> MSRGRKNNDIPLSFYNPITLEQGSKFWNLCP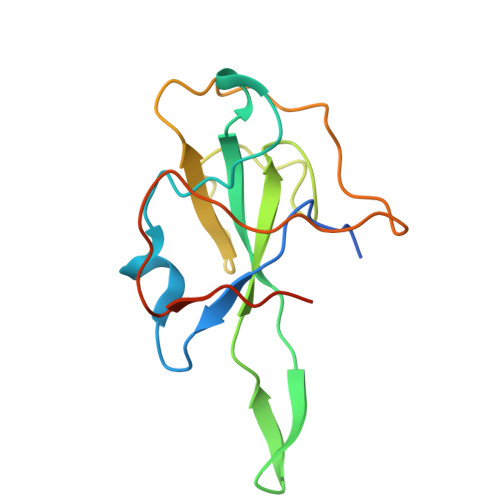RDLVPKGIGNKDQQIGYWNRQIRYRIVKGQRKELAERWFFYFLGTGPHADAKFKDKIDGVFWVARDGAMNKPITLGTRGTNNESKPLRFDGKIPPQFQLELEHHHHHHHH8-{[(2-cyanopyridin-3-yl)methyl]sulfanyl}-6-hydroxy-3,4-dihydro-1H-pyrano[3,4-c]pyridine-5-carbonitrile | C16 H12 N4 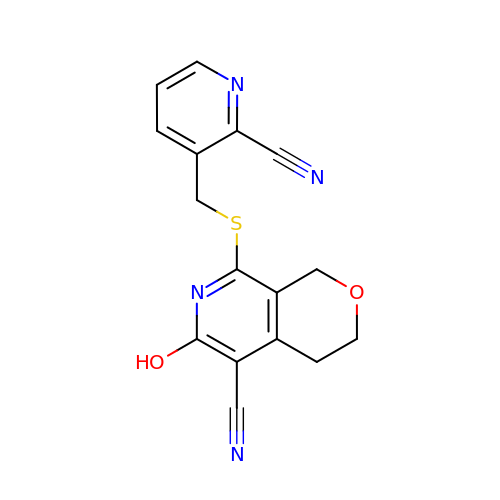O2 S | RMZOHPFYZBRDJW-UHFFFAOYSA-N>GSAKDPMHNFTYWNPTKLIFGRGEVERLPEELKSYGKNVLLVYGGGSIKRSGLYDQVIEQLNKAGVTVHELAGVEPNPRVSTVNKGVALCKEHHIDFLLAVGGGSVIDCTKAIAAGAKYDGDAWDIVTKKHQPKDALPFGTVLTLAATGSEMNSGSVITNWETKEKYGWGSPLVFPKFSILDPVNTFTVPKNHTIYGMVDMMSHVFEQYFHHVSNTPYQDRMCESLLRTVIETAPKLINDLENYELRETILYTGTIALNGMLSMGARGDWATHNIEHAVSAVYDIPHAGGLAILFPNWMRHTLSENPARMKQLAVRVFGVEEAGKTDKEVALEGIDKLSAFWTSLGAPNRLADYDINDEQLDTIADKAMANGTFGQFKSLNKEDVLAILKASL[2x]

Based on structural and biochemical studies, we report here that YugJ from B. subtilis is an atypical NADPH-dependent group III AAOR that reduces furan aldehyde in the presence of a Ni2+ cofactor. YugJ folds into a two-domain structure consisting of a Rossmann-like domain and an α-helical domain. YugJ interacts with NADP and Ni2+ using the interdomain cleft of YugJ. YugJ was highly active as an HMF reductase when supplemented with NADPH, but it was inactive with NADH, indicating that YugJ is an NADPH-dependent aldehyde reductase.

To obtain structural insights into YugJ-mediated aldehyde reduction, we determined the crystal structure of YugJ in complex with Ni2+ ions (YugJNi) at a 2.15 Å resolution in space group P212121 by molecular replacement. The asymmetric unit of the YugJ crystal contains two YugJ polypeptide chains (chains A and B), which are arranged into a homodimer. In the YugJNi structure, a strong electron density peak that belongs to a metal ion was found in each YugJ monomer, although a metal ion was not used for crystallization. In the spectrum, a prominent peak was observed at 7.46 keV, which corresponds to the X-ray emission energy of the Ni2+ ion, indicating that the metal ion observed in the YugJ structure is a Ni2+ ion. The Ni2+ ion is located between the two α-helix bundles of the CTD in the interdomain cleft and coordinated by conserved aspartate (Asp194) and histidine (His198, His267, and His281) residues. Given that YugJ exhibited high aldehyde reductase activity in the presence of Ni2+ ions and was observed with Ni2+ ions in the crystal structure of YugJNi, we conclude that YugJ is an atypical group III AAOR that favors a Ni2+ ion as a metallic cofactor. YugJ exhibits interdomain flexibility in the absence of NADP, given that YugJ chains A and B in the YugJNi structure adopt open and closed conformations, respectively, which differ in interdomain angle by ~10°. In contrast, the α9–α10 loop of the YugJNi and YugJNADP-Ni structures adopts an open conformation that increases the accessibly of the active site. Accordingly, an additional three-pointed density was not observed in the YugJNi or YugJNADP-Ni structure obtained in the absence of nitrate.(2R,4R)-2-methyl-1,3-thiazolidine-2,4-dicarboxylic 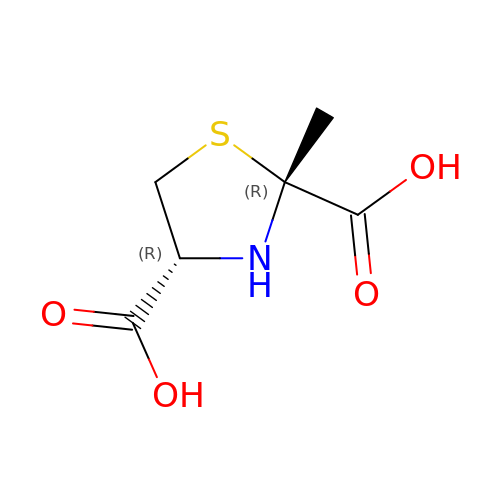acid | C6 H9 N O4 S | JCAKCGQZNBEITC-BBIVZNJYSA-N>MAASQTSQTVASHVPFADLCSTLERIQKSKGRAEKIRHFREFLDSWRK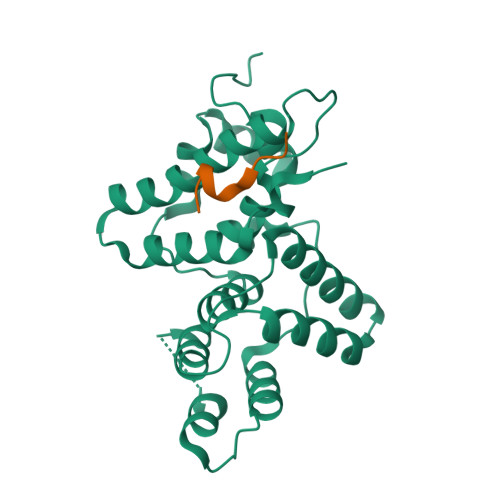FHDALHKNHKDVTDSFYPAMRLILPQLERERMAYGIKETMLAKLYIELLNLPRDGKDALKLLNYRTPTGTHGDAGDFAMIAYFVLKPRCLQKGSLTIQQVNDLLDSIASNNSAKRKDLIKKSLLQLITQSSALEQKWLIRMIIKDLKLGVSQQTIFSVFHNDAAELHNVTTDLEKVCRQLHDPSVGLSDISI[2x];>DVPQWEVFFKR[2x]> NECLVETRTTRISGRDALCVDVAGALTSDGSRLILYPCGQQVNQKWTFHSDGTVRSLGKCLATNNSKFGNLVVIYDCSKLAAEDISWDVSVGGTIMNPNYEDLALTSNKATRSTNLTMEVNTYSASQGWRVGNYVQPIIGSIVGLDDMCL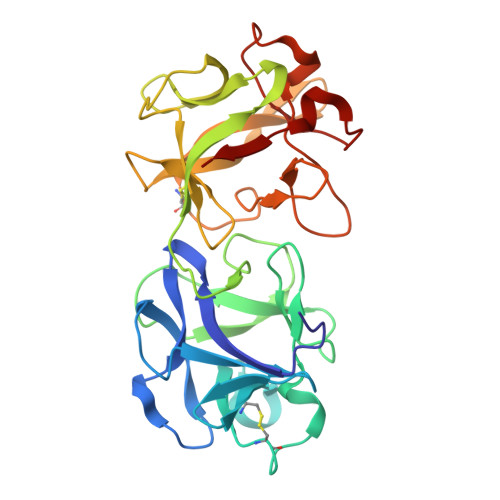EATDGNTNMWLEECVPNQREQSWALYSDGTIRVDDNRELCVTASSSTYDNWKVITILNCDGSNNQRWVFLADGSISTPGNQRLAMDVARSDVDLKKIILHRPHGDLNQQWVLFY> EAEATDPNGYIVFCPCMGRFGNQVDQFLGVLAFAKALDRTLVLPNFIEFKHPETKMIPFEFLFQVGTVAKYTRVVTMQEFTKKIMPTVWPPEKRKAFCWTPRQAIYDKSAEPGCHSKEGNPFGPYWDQIDVSFVGDEYFGDIPGGFDLNQMGSRKKWLEKFPSEEYPVLAFSSAPAPFPSKGKVWSIQKYLRWSSRITEQAKKFISANLAKPFVAVHLRNDADWVRVCEHIDTTTNRPLFASEQCLGEGHHLGTLTKEICSPSKQQILEQIVEKVGSIGAKSVFVASDKDHMIDEINEALKPYEIEAHRQEPDDMYTSLAIMGRADLFVGNCVSTFSHIVKRERDHAGQSPRPSAFFGIRAV

POFUT1 α-fucosylates serines or threonines present in EGF repeats containing the appropriate consensus sequence, C2-X(4-5)-[S/T]-C3, where C2 and C3 are the second and third conserved cysteines. In the present study we have solved the first crystal structure of CePOFUT1, which serves as a conserved family member. The protein shows a typical GT-B fold formed by two Rossmann domains. A cavity for GDP-fucose is localised in the interface between the domains and a contiguous solvent exposed pocket for EGF repeats was identified by electrostatic and docking studies.

The fourth one is a crystal-form-III in complex with GDP, resembling a product complex. The structures show the typical GT-B folding and a non-metal dependency. We also determined the activity of CePOFUT1 in the presence of 1 and 5 mM MnCl2, showing that the enzyme is inhibited by manganese (between 40–60% inhibition, data not shown), contrary to what has previously been described. CePOFUT1 is a catalytically competent non manganese-dependent enzyme, transfering fucose to MmEGF12. Unlike Asp242 or Asp244, Arg240 played an important key role in binding and catalysis. The role of Arg240 is crucial in order to stabilize the charge of the incipient free phosphate group thus promoting its dissociation from the anomeric center.Lamivudine Triphosphate 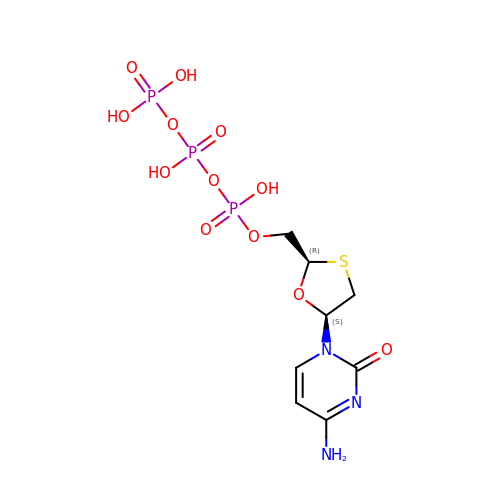| C8 H14 N3 O12 P3 S | YLEQMGZZMCJKCN-NKWVEPMBSA-N>GSHMNITVSGDSSQLQSGMGLDKLIDGTTSSDDSSRMDLKWIFTSDQQDKGTLPFEMTFEFNEPKTLENFTIYNRMNSNGTINIAAMKKVKAVGYLNGEEFDLGEKANITSATTVYELGGKEFDKIVITALDSHKDKNTLAINEIEFYEKSE[2x]

As part of the secreted C. perfringens CAZyme arsenal, the bacterium possesses an open reading frame coding for a 220-kDa family 31 glycoside hydrolase (locus tag CPF_1301 in strain ATCC 13124) with predicted α-glucosidase activity, which will be hereafter referred to as CpGH31. In addition to the N-terminal glycoside hydrolase family 31 catalytic module, CpGH31 comprises two fibronectin-type III modules, three CBM32s, a putative cohesin module, and a bacterial immunoglobulin-like 2 module. Though the putative CBMs, referred to as CBM32-1, CBM32-2, CBM32-3, themselves are not closely related at the amino acid sequence level, a primary structure comparison indicates that they all belong to CBM family 32, an observation that is supported by their overall similar structures as determined by X-ray crystallography. Each CpGH31 CBM32 structure comprised the β-sandwich topology characteristic of this CBM family with a short α-helix and a calcium ion capping one side of each module.

In contrast, CBM32-2 displayed a clear binding specificity for GalNAc. A structural rationale for the observed GalNAc specificity displayed by CpGH31 CBM32-2 was provided by the X-ray crystal structure of the CBM32-2:GalNAc complex determined to 2.0 Å. The GalNAc was well-ordered in the crystal structure and provided sufficiently clear electron density for modelling the monosaccharide into the binding site of CpGH31 CBM32-2. GalNAc was coordinated by a subset of residues located in the variable loop region at the apex of CBM32-2. The side chain of Trp1359 formed the main aromatic-based CH-π interaction between the b-face of GalNAc and the protein surface. Notably, the binding site lacked additional sugar-coordinating aromatic residues, which is an unusual feature among clostridial CBM32s that has only been previously observed in the non-canonical galactose-binding CpGH84A CBM32-1. With respect to the observed GalNAc specificity by CBM32-2, the shallow binding surface accommodated the hydroxyl O4 group of the sugar in the axial position only. As such, the topology of the binding site cannot accommodate gluco-configured ligands such as glucose, GlcNAc, or GlcN. In order to selectively bind GalNAc over other galacto-configured ligands (i.e., galactose and LacNAc), polar residues in the binding site were positioned to form water-mediated hydrogen bonding interactions to the 2-acetamido group in addition to the coordination of the O6 hydroxyl groups of the sugar. Since the hydrogen bonds involving the extended 2-acetamido group of GalNAc and the side chains of Asp1351, Arg1393 and Asn1401 were observed to be water-mediated, the distance between these side chains and the shorter O2 hydroxyl group of galactose or the galactose moiety of LacNAc may be too great to allow for these ligands to adhere to the protein surface.> GAVFIFVGAL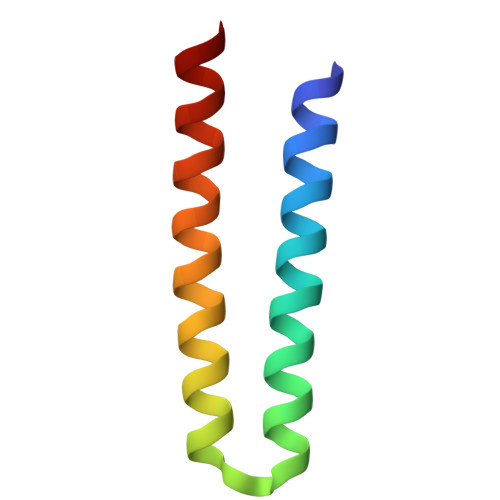TVLFGAIAYGEVTAAAATGDAAAVQEAAVSAILGLIILLGINLGLVAATL>MAFSDLTSRTVHLYDNWIKDADPRVEDWLLMSSPLPQTILLGFYVYFVTSLGPKLMENRKPFELKKAMITYNFFIVLFSVYMCYEFVMSGWGIGYSFRCDIVDYSRSPTALRMARTCWLYYFSKFIELLDTIFFVLRKKNSQVTFLHVFHHTIMPWTWWFGVKFAAGGLGTFHALLNTAVHVVMYSYYGLSALGPAYQKYLWWKKYLTSLQLVQFVIVAIHISQFFFMEDCKYQFPVFACIIMSYSFMFLLLFLHFWYRAYTKGQRLPKTVKNG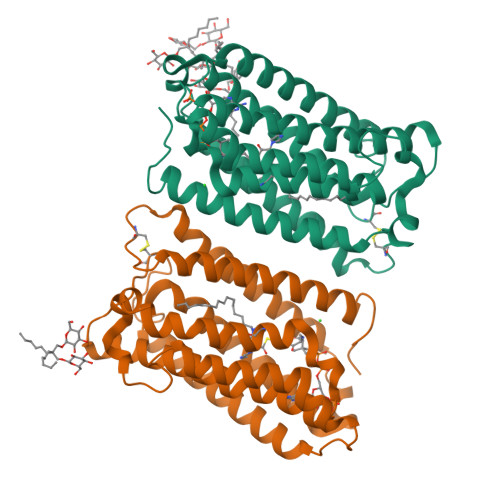TCKNKDNAENLYFQ[2x]> DLGSFKANFIDSDGNQMTDVVEINFADATEKNISNLLNTLLGRDREEFTPYRFRIHIPGKDLIIDQYPNDLLSLLQKHGVTNPFETTITLSAEPQAIFKVHAVSRLAHRIPGHGQPILSCQFSPVSSSRLATGSGDNTARIWDTDSGTPKFTLKGHTGWVLGVSWSPDGKYLATCSMDTTVRVWDPESGKQVNQEFRGHAKWVLALAWQPYHLWRDGTARLASASKDCTVRIWLVNTG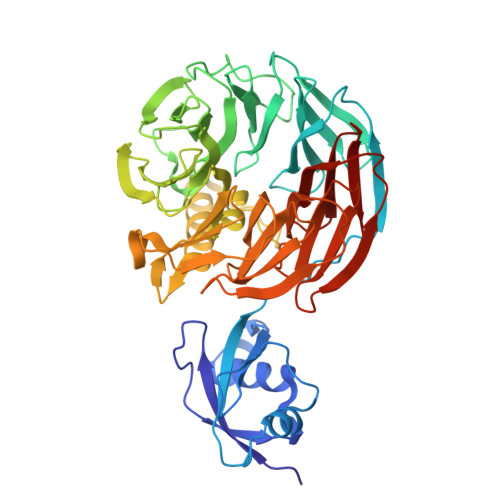RTEHVLSGHKGSVSCVKWGGTDLIYTGSHDRSVRVWDAVKGTLVHNFTAHGHWVNHIALSSDHVLRTAYHDHTKEVPGTEEERRAKAKERFEKAAKIKGKVAERLVSASDDFTMYLWDPTNNGSKPVARLLGHQNKVNHVQFSPDGTLIASAGWDNSTKLWNARDGKFIKNLRGHVAPVYQCAWSADSRLVVTGSKDCTLKVWNVRTGKLAMDLPGHEDEVYAVDWAADGELVASGGKDKAVRTWRN>MAGAEWKSLEECLEKHLPLPDLQEVKRVLYGKELRKLDLPREAFEAASREDFELQGYAFEAAEEQLRRPRIVHVGLVQNRIPLPANAPVAEQVSALHRRIKAIVEVAAMCGVNIICFQEAWTMPFAFCTREKLPWTEFAESAEDGPTTRFCQKLAKNHDMVVVSPILERDSEHGDVLWNTAVVISNSGAVLGKTRKNHIPRVGDFNESTYYMEGNLGHPVFQTQFGRIAVNICYGRHHPLNWLMYSINGAEIIFNPSATIGALSESLWPIEARNAAIANHCFTCAINRVGTEHFPNEFTSGDGKKAHQDFGYFYGSSYVAAPDSSRTPGLSRSRDGLLVAKLDLNLCQQVND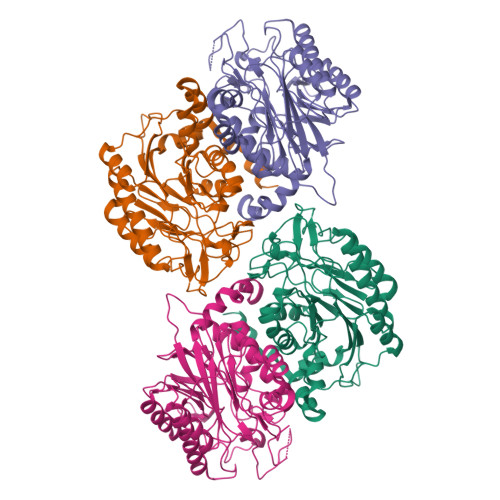VWNFKMTGRYEMYARELAEAVKSNYSPTIVKE[4x]(3AR,5R,6S,7R,7AR)-2,5-BIS(HYDROXYMETHYL)-5,6,7,7A-TETRAHYDRO-3AH-PYRANO[3,2-D][1,3]OXAZOLE-6,7-DIOL | C8 H13 N O6 | 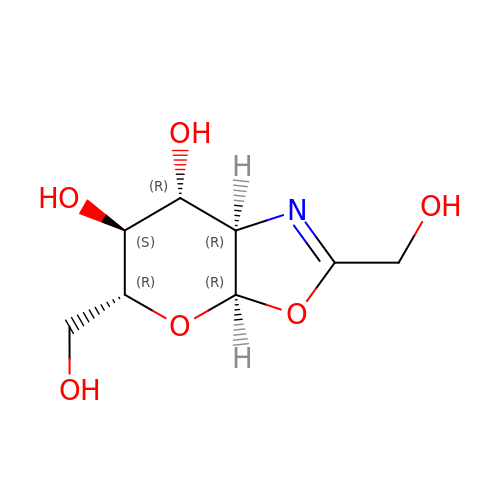FAUNLXBEFZYFSG-PNAXYBNRSA-N>MGRGKVKPNRKSTGDNSNVVTMIRAGSYPKVNPTPTWVRAIPFEVSVQSGIAFKVPVGSLFSANFRTDSFTSVTVMSVRAWTQLTPPVNEYSFVRLKPLFKTGDSTEEFEGR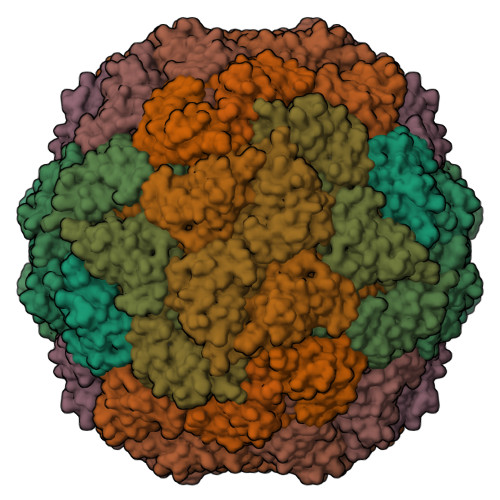ASNINTRASVGYRIPTNLRQNTVAADNVCEVRSNCRQVALVISCCFN[15x]> AMAAKVVYVFSTEMANKAAEAVLKG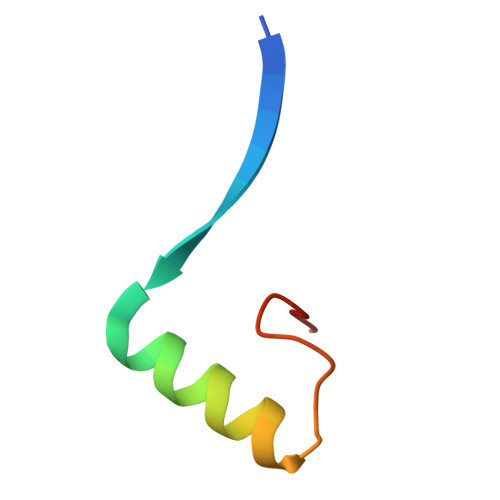QVETIVSFHI> MAILDVDTVYTNTGDILQIGYAQKAADNGNTAICMKNKKGLIMIAEKPIESKLYVSEKNFRIKKVNNSIFQISSGIETDLVYINENLKNNLISEKHSNDMDVSHESVRNQIVNIIHQFTRYSGVRPIGINLLTCSKYKNEYKILQTDCTGKSLFFKS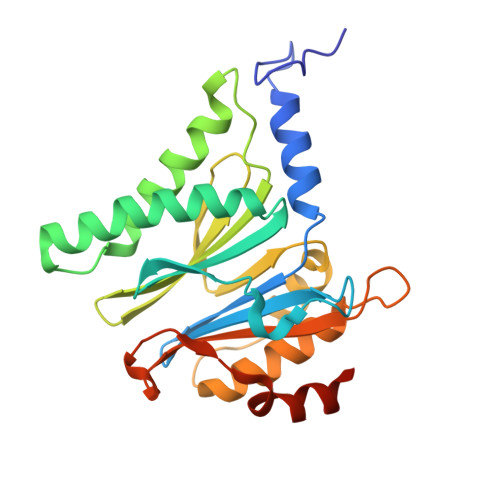SVIGKGSRIVKTELEKLNLENMEIRDLVENGIRILYKSYDPLKDKPFDIEIGIMCEETNGEFVRLEKNQYSEIIEKYKDFSVDGEE>VIHNESTCEQLAKANAGKPKDPTFIPAPIQAKTSPVDEKALQDQLVLVAAKLDTEDKLRAAMVGMLANFLGFRIYGMHSELWGVVHGATVLSPTAVFGTLASLYLGALDHTADRLQAILGVPWKDKQCTSRLDAHKVLSALQAVQGLLVAQGRADSQAQLLLSTVVGVFTAPGLHLKQPFVQGLALYTPVVLPRSLDFTELDVAAEKIDRFMQAVTGWKTGSSLMGASVDSTLAFNTYVHFQGKMKGFSLLAEPQEFWVDQSTSVSVPMLSGMGTFQHWSDIQDQFSVTQVPFTESASLLLIQPHYASDLDKVEGLTFQQNSLNWMKKLSPRTIHLTMPQLVLQGSYDLQDLLAQAELPAILHTELNLQKLSNDRIRVGEVLNSIFFELEADEREPTESTQQLNKPEVLEVTLNRPFLFAVYDQSATALHFLGRVANPLSTAHHHHHH[2x]

Human blood pressure is mainly controlled by the renin–angiotensin system, which consists of several key components, including renin, angiotensinogen (AGT),3 angiotensin-converting enzyme (ACE), and angiotensin receptors. Renin is a highly specific aspartic protease that cleaves AGT between Leu10 and Val11 to release the N-terminal angiotensin I peptide. Cleavage of AGT by renin is the rate-limiting step of the renin–angiotensin system. To address these questions, here we have solved high-resolution crystal structures of human glycosylated AGT, its encounter complex with renin, AGT cleaved in the reactive center loop, and the spent AGT from which the N-terminal angiotensin peptide has been removed by renin.

To further dissect the conformational plasticity of AGT, we then solved the crystal structure of spent AGT and compared it with that of intact AGT. The spent AGT retains a fold similar to that of native AGT with an r.m.s. deviation of 0.63 Å over 355 Cα atoms. Helices A, I, and J of spent AGT, which are involved in renin binding, have the same conformation as in native AGT. In contrast, there are significant movements in the CD-loop. However, it is notable that the rearrangement of the CD-loop in spent AGT places the side chain of Trp133 in the hydrophobic pocket occupied by the scissile peptide region in intact AGT, replacing the side chain of Val11. Finally, helix H in the spent human AGT is disordered with no clear electron density, whereas it is in a helical conformation in intact AGT. This may also be influenced by crystal packing; if helix H in spent AGT were ordered in the same conformation as in intact AGT, it would clash with the CD-loop of a neighboring molecule. A reduced stability of helix H in spent AGT could partly explain why spent AGT only has a relatively low binding affinity toward renin. The binding affinity derived from steady-state analysis gives a KD value of 13 μm, which is 640-fold weaker than the binding of intact AGT to renin. Therefore, we conclude that spent AGT does have a product inhibition effect on renin cleavage of intact AGT; however, it is unlikely to be significant in vivo.5'-O-(D-valylsulfamoyl)adenosine | C15 H23 N7 O7 S | 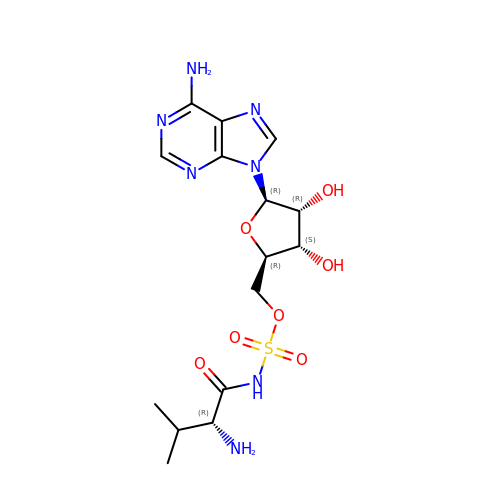TXCZGHBHNXNXMA-FGOODDOWSA-N> FTTGLVYDTLMLKHQCTCGSSSSHPEHAGRIQSIWSRLQETGLRGKCECIRGRKATLEELQTVHSEAHTLLYGTNPLNRQKLDSKKLLGSLASVFVRLPCGGVGVDSDTIWNEVHSAGAARLAVGCVVELVFKVATGELKNGFAVVRPPGHHAEESTPMGFCYFNSVAVAAKLLQQRLSVSKILIVDWD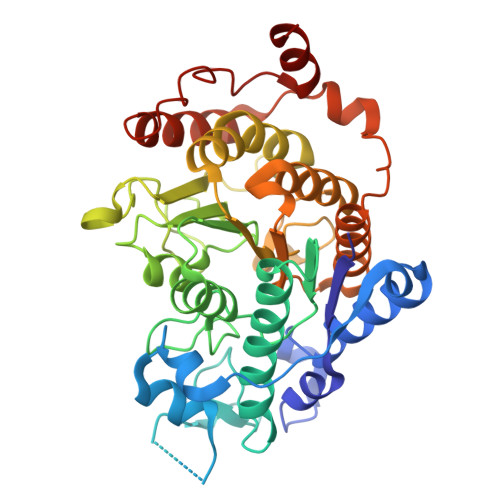VHHGNGTQQAFYSDPSVLYMSLHRYDDGNFFPGSGAPDEVGTGPGVGFNVNMAFTGGLDPPMGDAEYLAAFRTVVMPIASEFAPDVVLVSSGFDAVEGHPTPLGGYNLSARCFGYLTKQLMGLAGGRIVLALEGGYDLTAICDASEACVSALLGNELDPLPEKVLQQRPNANAVRSMEKVMEIHSKYWRCLQRTTSTAGRSLIEAQTCEN>SNAMKKFLGAYQNNHMHWVGDGFPVYNLFSYDRLGQTLSPFLLLDYAAPYNFSPTTEQQGVGSHPHRGFETVTIAYQGEVTH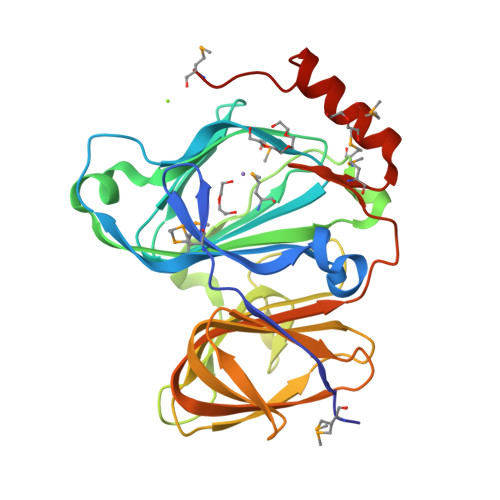KDSSGGGGTIKTGDVQWMTAGAGVLHEEFHSPEFAEHGGLFEMVQLWVNLPSHSKMTPGKYQAIEAKDIPDIALDEHGSHLRVIAGEYADAKGAATTFSPLNVWDGKLVKGQKHTLYVPEGHTTLVVVLEGAVVVNDTNRLEGKTVAILSREGVEFSLNAEEDTKFLVLTGQPLNEPIEGYGPFVMNTKAEIMEAINDFNRGKFGSIMQEG[4x]>[2x]AFLHVGAQLGTELFIVRQLLQIVKQKTNQNSVDTTLKFTLSALWNLTDESPTTCRHFIENQGLELFMRVLESFPTESSIQQKVLGLLNNIAEVQELHSELMWKDFIDHISSLLHSVEVEVSYFAAGIIAHLISRGEQAWTLSRSQRNSLLDDLHSAILKWPTPECEMVAYRSFNPFFPLLGCFTTPGVQLWAVWAMQHVCSKNPSRYCSMLIEEGGLQHLYNIKDHEHTDPHVQQIAVAILDSLEKHIVR

ZER1 and ZYG11B, the substrate receptors of the Cullin 2-RING E3 ubiquitin ligase (CRL2), recognize N-terminal (Nt) glycine degrons and participate in the Nt-myristoylation quality control through the Gly/N-degron pathway. Here we show that ZER1 and ZYG11B can also recognize small Nt-residues other than glycine. Furthermore, we present the crystal structures of ZER1 and ZYG11B bound to various small Nt-residues and uncover the molecular mechanism of non-acetylated substrate recognition by ZER1 and ZYG11B. In conclusion, we propose that ZER1/ZYG11B not only targets Gly/N-degrons for proteasomal degradation, but it also has the ability to bind a defined selection of non-Ac/N-degrons by a conserved molecular mechanism of substrate recognition and target their degradation through the non-Ac/N-degron pathway.

To understand the molecular basis of ZER1/ZYG11B-mediated binding of non-Gly Nt-residue peptides, we determined the crystal structures of ZER1 bound to either SFLH-, AFLH- or TFLH-peptide, as well as the crystal structures of ZYG11B bound to either SFLH-, AFLH- or CFLH- peptide. Meanwhile, ZYG11B displayed appreciable binding to Nt-Ser (KD of 6.8), -Ala (KD of 7.1), or -Cys (KD of 3.0), albeit slightly weaker than Nt-Gly (KD of 2.5). Structural comparisons indicated that the peptide-binding modes of ZER1 and ZYG11B are similar. The free α-amino group of the Nt-residue forms hydrogen bonds with the side chains of Asp556 and Asn597 in ZER1 (the counterparts of Asp 526 and Asn 567 in ZYG11B), respectively. Furthermore, the carbonyl oxygen of the Nt-residue is stabilized by two hydrogen bonds from Asn597 and Trp552 in ZER1 (Asp 567 and Trp522 in ZYG11B). The main-chain amide and carbonyl of the second residue (F2) on the peptide hydrogen bond to the main-chain respective carbonyl and amide of Asn679 in ZER1 (Ala647 in ZYG11B). The main-chain amide of the third residue on the peptide is anchored by a hydrogen bond with Asn553 in ZER1 (Asn523 in ZYG11B). Likewise, consistent with the structural observations, the mutants W522A, D526A, N567A, E570A and N523A in ZYG11B were defective in binding to the XFLHVGQD (X = Ser, Ala or Cys) peptides.> GAACAUAUAAUCG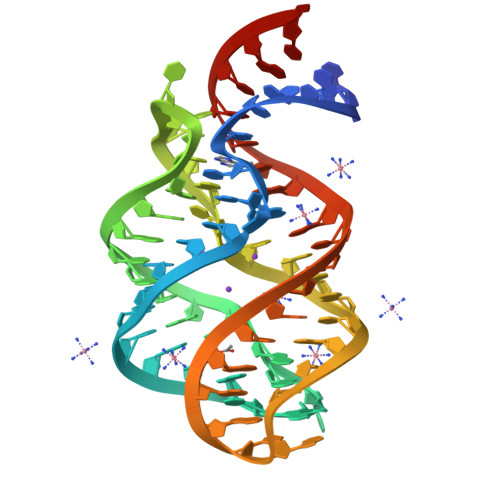CGUGGAUAUGGCACGCAAGUUUCUACCGGGCACCGUAAAUGUCCGAUUAUGUCC> FMFKHIIARTPARSLVDGLTSSHLGKPDYAKALEQHNAYIRALQTCDVDITLLPPDERFPDSVFVEDPVLCTSRCAIITRPGAESRRGETEIIEETVQRFYPGKVERIEAPGTVEAGDIMMVGDHFYIGESARTNAEGARQMIAILEKHGLSGSVVRLEKVLHLKTGLAYLEHNNLLAAGEFVSKPEFQD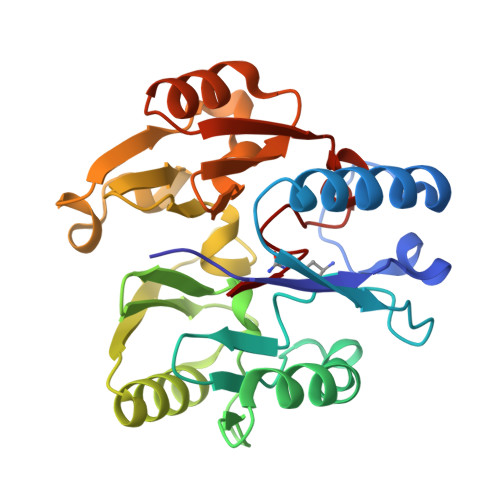FNIIEIPEEESYAANCIWVNERVIMPAGYPRTREKIARLGYRVIEVDTSEYRKIDGGVSSMSLRF> AVSKVYARSVYDSRGNPTVEVELTTEKGVFRSIVPSGASTGVHEALEMRDGDKSKWMGKGVLHAVKNVNDVIAPAFVKADIDVKDQKAVDDFLISLDGTANKSKLGANAIL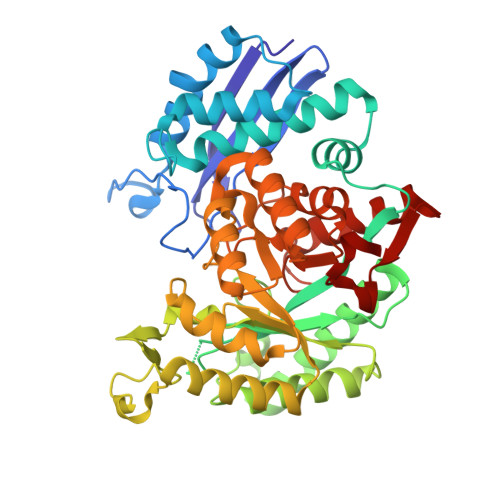GVSLAASRAAAAEKDVPLYKHLADLSKSKTSPYVLPVPFLNVLNGGSHAGGALALQEFMIAPTGAKTFAEALRIGSEVYHNLKSLTKKRYGASAGNVGDEGGVAPNIQTAEEALDLIVDAIKAAGHDGKVKIGLDCASSEFFKDGKYDLDFKNPNSDKSKWLTGPQLADLYHSLMKRYPIVSIEDPFAEDDWEAWSHFFKTAGIQIVADDLTVTNPKRIATAIEKKAADALLLKVNQIGTLSESIKAAQDSFAAGWGVMVSHRSGETEDTFIADLVVGLRTGQIKTGAPARSERLAKLNQLLRIEEELGDNAVFAGENFHHGDKL> SIPWNLE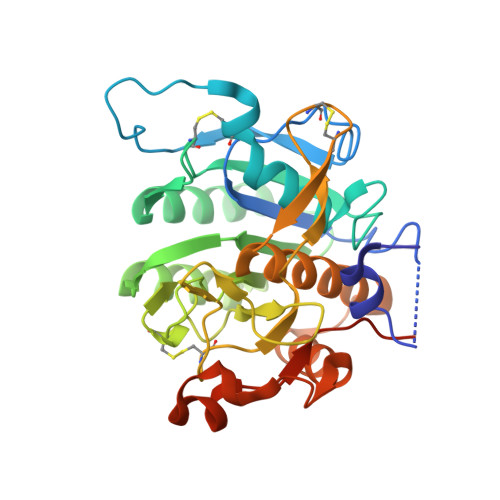RITPPRYRADEYQPPDGGSLVEVYLLDTSIQSDHREIEGRVMVTDFENVPEEDGTRFHRQASKCDSHGTHLAGVVSGRDAGVAKGASMRSLRVLNCQGKGTVSGTLIGLEFIRKSQLVQPVGPLVVLLPLAGGYSRVLNAACQRLARAGVVLVTAAGNFRDDACLYSPASAPEVITVGATNAQDQPVTLGTLGTNFGRCVDLFAPGEDIIGASSDCSTCFVSQSGTSQAAAHVAGIAAMMLSAEPELTLAELRQRLIHFSAKDVINEAWFPEDQRVLTPNLVAALPPSTHGAGNSHHHHHH>[2x]SSSYTEADPAILSRRQKQIDYGKNTAAYERYVEMVPKDERTRDHPRE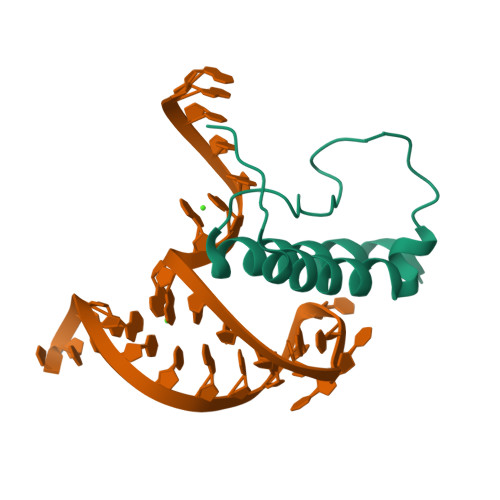PNKYGKYSRRAFDGLVKIWRKSLHIYDPPTQARDTAKDENEDEDED>[2x]APQQINDIVHRTITPLIEQQKIPGMAVAVIYQGKPYYFTWGYADIAKKQPVTQQTLFELGSVSKTFTGVLGGDAIARGEIKLSDP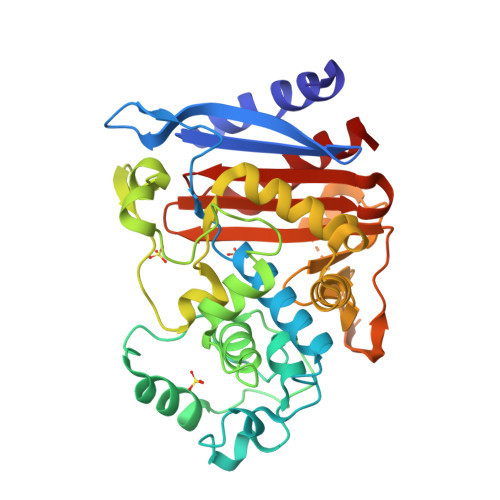TTKYWPELTAKQWNGITLLHLATYTAGGLPLQVPDEVKSSSDLLRFYQNWQPAWAPGTQRLYANSSIGLFGALAVKPSGLSFEQAMQTRVFQPLKLNHTWINVPPAEEKNYAWGYREGKAVHVSPGALDAEAYGVKSTIEDMARWVQSNLKPLDINEKTLQQGIQLAQSRYWQTGDMYQGLGWEMLDWPVNPDSIINGSDNKIALAARPEKAITPPTPAVRASWVHKTGATGGFGSYVAFIPEKELGIVMLANKNYPNPARVDAAWQILNALQ> GPHMSVSESAVFAYESSVHSTNVLLSLNDQRKKDVLCDVTV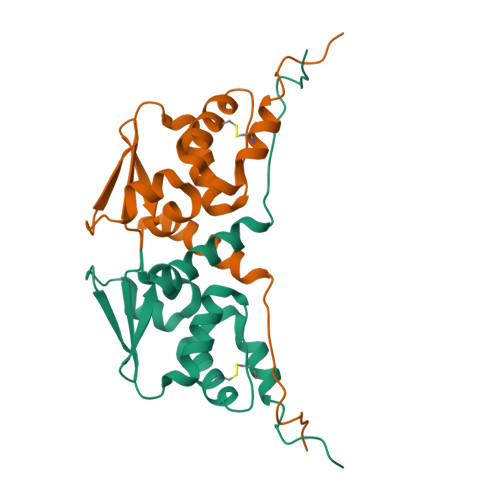LVEGQRFRAHRSVLAACSSYFHSRIVGQTDAELTVTLPEEVTVKGFEPLIQFAYTAKLILSKDNVDEVCRCVEFLSVHNIEESCFQFLKFKFLDSTS>GSNPTRSIPATDAVSSATAGKKMGLQTYSLGQELLQDMPNGLNRLAKAGYTDLEIFGYREDTGKFGDYNPKNTTFIASKDYKKMVDDAGLRISSSHLTPSLREYTKENMPKFDEFWKKATDIHAELGVSCMVQPSLPRIENEDDAKVVSEIFNRAGEITKKAGILWGYHNHSNEFKRVLKAGEKPEQNPNPWAPPKGTYIEELFLKNTDPDKVMFELDVYWAVMGQQDPVEWMENYPNRFKLLHIKDRWIIGDS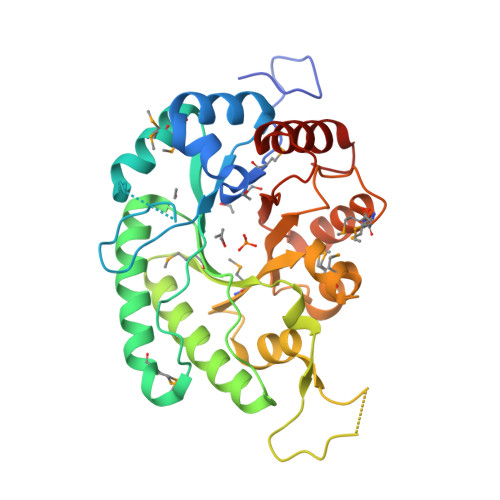GMMNFPNIFKKAYEIGILGYYVELEGDKKGRTQFEGVEKSAAYLQAAPFVK[2x]>STLADQALHNNNVGPIIRAGDLVEPVIETAEIDNPGKEITVEDRRAYVRIAAEGELILTRKTLEEQLGRPFNMQELEINLASFAGQIQADEDQ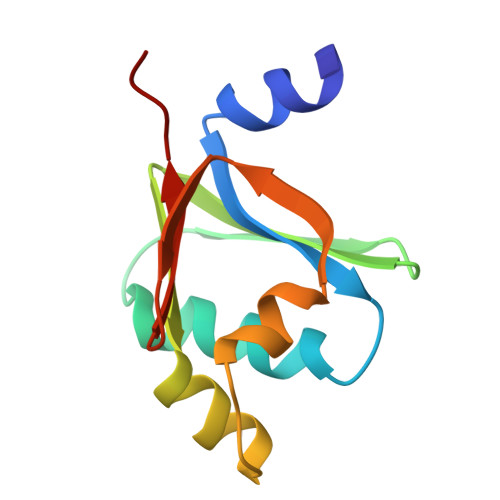IRFYFDKTM[2x]2-nitrophenyl beta-D-fucopyranoside | C12 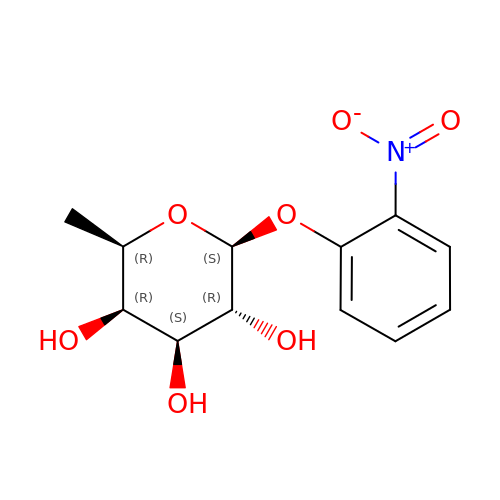H15 N O7 | SWRPIVXPHLYETN-BVWHHUJWSA-N>[2x]MGPVWRKHYITYRINNYTPDMNREDVDYAIRKAFQVWSNVTPLKFSKINTGMADILVVFARGAHGDDHAFDGKGGILAHAFGPGSGIGGDAHFDEDEFWTTHSG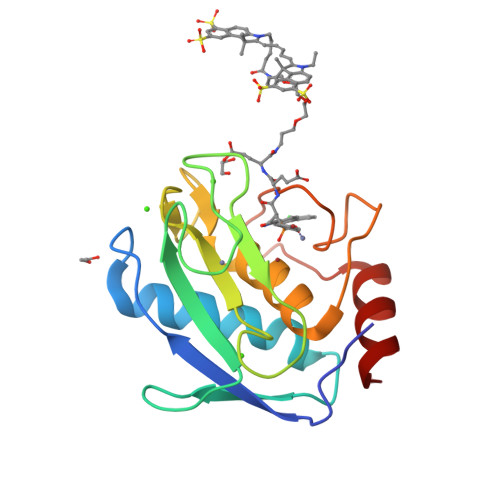GTNLFLTAVHEIGHSLGLGHSSDPKAVMFPTYAYVDINTFRLSADDIRGIQSLYG> PGGTRIIYDRKFLME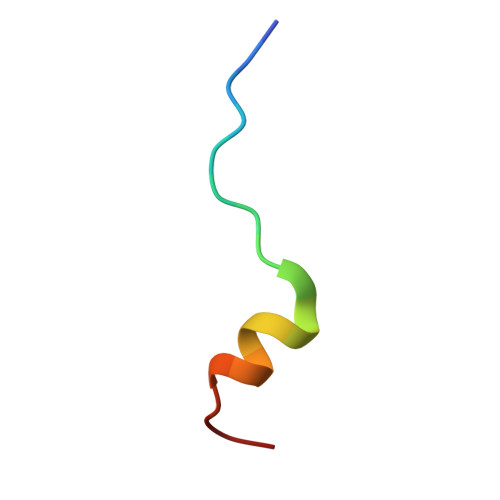CRNSP N-[3-[(1-AMINOETHYL)(HYDROXY)PHOSPHORYL]-2-(1,1'-BIPHENYL-4-YLMETHYL)PROPANOYL]ALANINE | C21 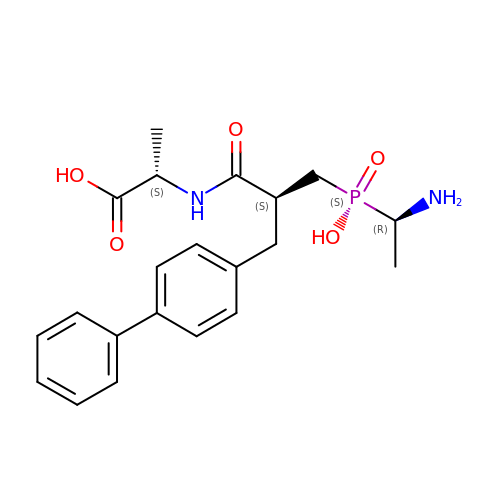H27 N2 O5 P | CWJPVKSBGVPXRD-QMTMVMCOSA-N>GSHMVAAGDNKIKQGLLPSLEDLLFYTIAEGQEKIPVHKFITALKSTGLRTSDPRLKECMDMLRLTLQTTSDGVMLDKDLFKKCVQSNIVLLTQAFRRKFVIPDFMSFTSHIDELYESAKKQSGGKVADYIPQLAKFSPDLWGVSVCTVDGQRHSIGDTKVPFCLQSCVKPLKYAIAVNDLGTEYVHRYVGKEPSGLRFNKLFLNEDDKPHNPMVNAGAIVVTSLIKQGVNNAEKFDYVMQFLNKMAGNEYVGFSNATFQSERESGDRNFAIGYYLKEKKCFPEGTDMVGILDFYFQLCSIEVTCESASVMAATLANGGFCPITGERVLSPEAVRNTLSLMHS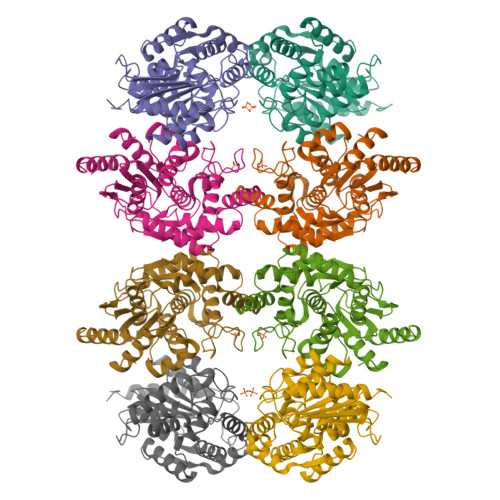CGMYDFSGQFAFHVGLPAKSGVAGGILLVVPNVMGMMCWSPPLDKMGNSVKGIHFCHDLVSLCNFHNYDNLRHFAKKLDPRREGGDQRHSFGPLDYESLQQELALKDTVWKKVSPESSDDTSTTVVYRMESLGERS[8x]>[6x]MEYELLIREAEPKD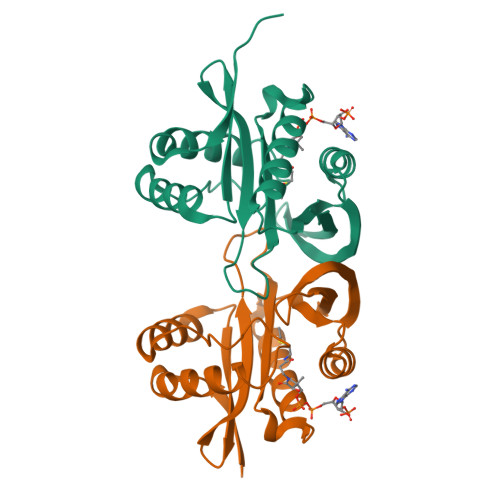AAELVAFLNRVSLETDFTSLDGDGILLTSEEMEIFLNKQASSDNQITLLAFLNGKIAGIVNITADQRKRVRHIGDLFIVIGKRYWNNGLGSLLLEEAIEWAQASGILRRLQLTVQTRNQAAVHLYQKHGFVIEGSQERGAYIEEGKFIDVYLMGKLIG>MSRPSVAIVSPAVASANNGNWQTARRWQEFLDGTCNVRMTQRWPDDGSQDDVVMLALHARRSADSIEAWASVHGDRGLAVVLTGTDLYQDIVVDPRARHSLELAGQLVVLQDLGAEALPPALRGKTRVIYQSTPSQAAASKPDTVLQALMVGHLREVKSPQTLFQAARLLAGHDDIRIDHIGEALDPVLGEQALATQRDCPNYRWLGALPHDGTRERIRCAHLLVHASAMEGGAHVIMEAVCSGTPVLASRIPGNVGMLGADYAGYFTHGDAAALAALL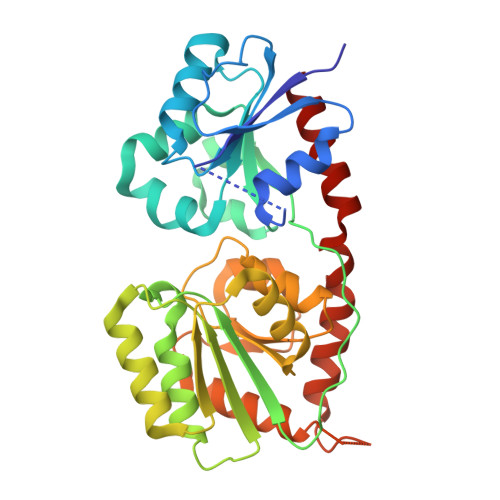VRCRQGQAASGDVPADPLLARLGAQCALRAPLFAPEAERAALLRLVADLM[2x]>[2x]REFMAVTANNSQLLTWWHNTGEINTQTPVADGNVRQSGLYSVKVQTTPASSSLYYDSFVYLAIPGNGMSDQLQYTQGYNQTQAWTSFLYSHDATVKISRNGSSANSNVVIRPTSLNFPVRYDNQSVYITVPYSPTGYRFSVEFDDDLISLAPSGARQPENALLIFASPFENSSTKPQPGSPNSIAPAPGRVLGLNTTSASTVVFNPGVYYFTGHDHMVLSSSVTWVYFAPGAYVKGAVEFLSTASEVKASGHGVLSGEQYVWYADPDEGYQKASGANNNGLRMWRGTLGNSSQTFVLNGVTVSAPPFNSMDWSGNSLDLITCRVDDYKQVGAFYGQTDGLEMYPGTILQDVFYHTDDDGLKMYYSNVTARNIVMWKES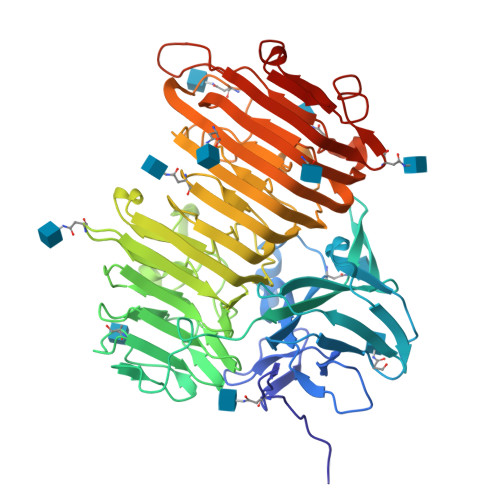VAPVVEFGWTPRNTENVLFDNVDVIHQAYANAGNNPGIFGAVNNYLYAPDGLSSNHSTGNSNMTVRNITWSNFRAEGSSSALFRINPIQNLDNISIKNVSIESFEPLSINTTESWMPVWYDLNNGKQITVTDFSIEGFTVGNTTITASNAASVGRIDGVDPAYAGSVHYID> GSHMGVEEPVYDATGKPLFGDPSEVHPQSTLKLPHDRGRGNIKTTLKNLPRKGDCRSGNHLGPVSGIYVKPGPVFYQDYMGPVYHRAPLEFFSEAQFCEVTKRIGRVTGSDGRLYHIYVCIDGCILLKLAKRGEPRTLKWIRNFTDCPLWVTSA

Pestiviruses, such as bovine viral diarrhea virus (BVDV) and classical swine fever virus (CSFV) use a virally encoded protein, the N-terminal protease (Npro), to suppress the transcriptional activation of the IFN-α/β genes by interacting with IRF3 and inducing its ubiquitination and proteasome-dependent degradation. The Npro protein is a leader cysteine autoprotease that cleaves itself from the nascent polyprotein during translation of the viral mRNA, freeing itself for innate immune suppression activities. Npro has a unique ‘clam shell’-like protease fold that is distinct from other known proteins including all known proteases. As predicted, Npro consists of two domains, a cysteine protease domain and a zinc-binding domain.

Here, we report the crystal structures of CSFV Npro and a C168A cleavage site Npro mutant to 1.6 Å resolution. The C168A protein was expressed as Npro-Δ17N protein that contains a Cys168 to Ala mutation along with an additional four residues at the C-terminus, 169Ser-Asp-Asp-Gly172, a sequence that corresponds to the first four amino acids of the core protein. This construct was intended to trap a substrate-bound form of Npro; by mutating the cleavage-site residue, Npro should not be able to catalyze self-cleavage at its C-terminus. Unexpectedly, the C168A mutant was active and the SDDG peptide at the C-terminus was cleaved, as confirmed by mass spectrometry (data not shown). Introduction of the Cys168 to Ala mutation resulted in different packing in the crystal lattice. The C168A Npro crystals belong to the spacegroup P212121 with one molecule per asymmetric unit and a solvent content of 54%. In comparison, CSFV Npro structures do not have a disulfide bond between Cys69 and Cys168 because the active site-containing helix is disordered in the wild-type Npro and Cys168 is replaced in the C168A Npro. Since C168A is as active as the wild-type Npro in our hands, disulfide bond formation is not a required step in catalysis. Thus, although Npro does not require Cys at the cleavage site, Cys168 is conserved in pestiviruses, suggesting that the residue may have an additional function other than participating in the protease catalysis.>LTGPLMLDTAPNAFDDQYEGCVNKMEEKAPLLLQEDFNMNAKLKVAWEEAKKRWNNIKPSRSYPKGFNDFHGTALVAYTGSIAVDFNRAVREFKENPGQFHYKAFHYYLTRALQLLSNGDCHSVYRGTKTRFHYTGA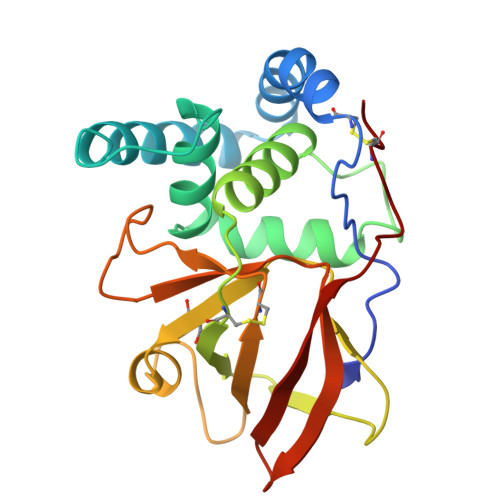GSVRFGQFTSSSLSKKVAQSQEFFSDHGTLFIIKTCLGVYIKEFSFRPDQEEVLIPGYEVYQKVRTQGYNEIFLDSPKRKKSNYNCLYS[2x]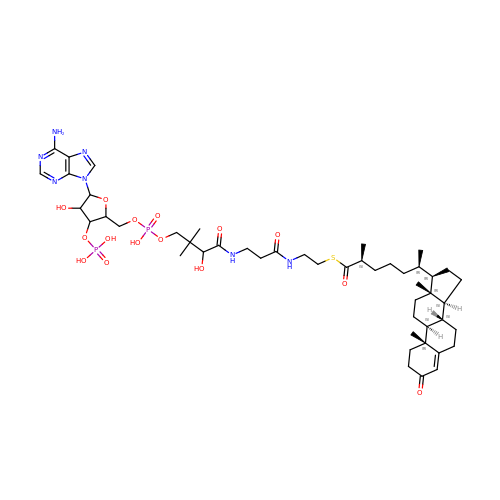S-{1-[5-(6-amino-9H-purin-9-yl)-4-hydroxy-3-(phosphonooxy)tetrahydrofuran-2-yl]-3,7-dihydroxy-6,6-dimethyl-3-oxido-8,12-dioxo-2,4-dioxa-9,13-diaza-3lambda~5~-phosphapentadecan-15-yl} (2S,6R)-6-[(8S,9S,10R,13R,14S,17R)-10,13-dimethyl-3-oxo-2,3,6,7,8,9,10,11,12,13,14,15,16,17-tetradecahydro-1H-cyclopenta[a]phenanthren-17-yl]-2-methylheptanethioate (non-preferred name) | C48 H75 N7 O15 P2 S | VHFLMCCTKSGQAT-YKQRDCBHSA-N>[2x]MSQTNANDLRNNEVFF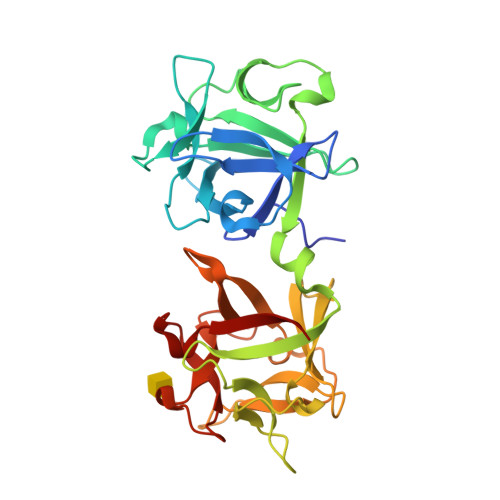ISPSNNTNKVLDKISQSEVKLWNKLSGANQKWRLIYDTNKQAYKIKVMDNTSLILTWNAPLSSVSVKTDTNGDNQYWYLLQNYISRNVIIRNYMNPNLVLQYNIDDTLMVSTQTSSSNQFFKFSNCIYEALNNRNCKLQTQLNSDRFLSKNLNSQIIVLWQWFDSSRQKWIIEYNETKSAYTLKCQENNRYLTWIQNSNNYVETYQSTDSLIQYWNINYLDNDASKYILYNLQDTNRVLDVYNSQIANGTHVIVDSYHGNTNQQWIINLI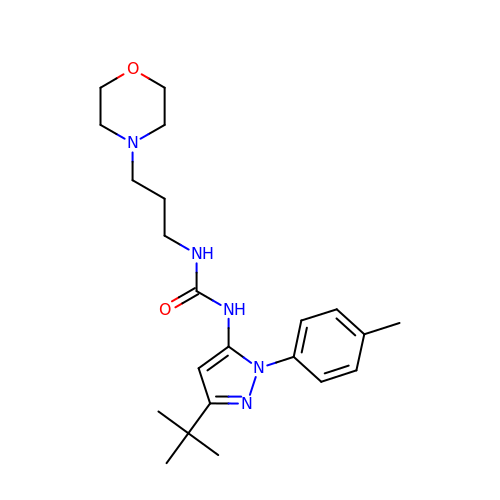1-[3-tert-butyl-1-(4-methylphenyl)-1H-pyrazol-5-yl]-3-[3-(morpholin-4-yl)propyl]urea | C22 H33 N5 O2 | LCMQASKUJYHHDV-UHFFFAOYSA-N> GSHMASPNGQTKPLPALKLALEYIVPCMNKHGICVVDDFLGKETGQQIGDEVRALHDTGKFTDGQLVSQKSDSSKDIRGDK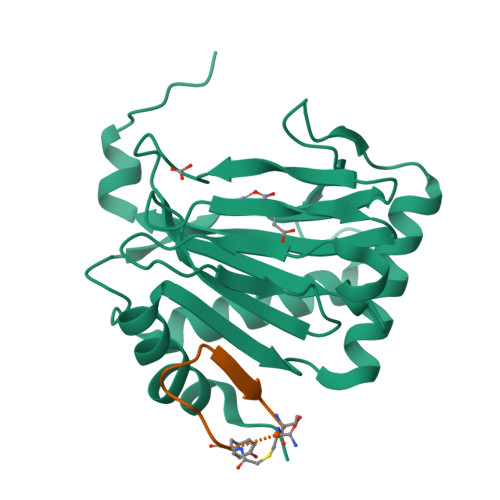ITWIEGKEPGCETIGLLMSSMDDLIRHCNGKLGSYKINGRTKAMVACYPGNGTGYVRHVDNPNGDGRCVTCIYYLNKDWDAKVSGGILRIFPEGKAQFADIEPKFDRLLFFWSDRRNPHEVQPAYATRYAITVWYFDADERARAKVKYLTGE;> XYVWLTDTWVLSRT>[2x]SPYSSDTTP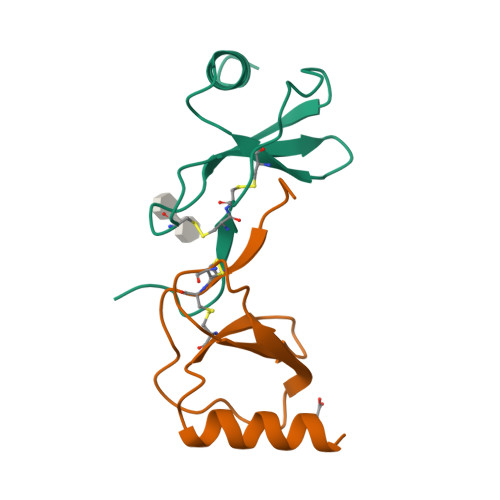CCFAYIARPLPRAHIKEYFYTSGKCSNPAVVFVTRKNRQVCANPEKKWVREYINSLEMS> STE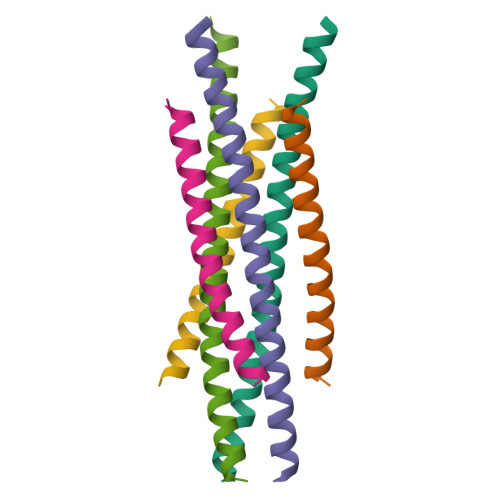NLYFQSNADSVQNHTFEVENNTINGLELTEEQVHILYAMVLQTHADVQLLKEQQ;> TQWDDWVDKMENLNHDILTTLHTARNNLEQSMITFNT>MGHHHHHHENLYFQGHFVQQKVKVFRAADPLVGVFLWGVAHSINELSQVPPPVMLLPDDFKASSKIKVNNHLFHRENLPSHFKFKEYCPQVFRNLRDRFGIDDQDYLVSLTRNPPSESEGSDGRFLISYDRTLVIKEVSSEDIADMHSNLSNYHQYIVKCHGNTLLPQFLGMYRVSVDNEDSYMLVMRNMFSHRLPVHRKYDLKGSLVSREASDKEKVKELPTLKDMDFLNKNQKVYIGEEEKKIFLEKLKRDVEFLVQLKIMDYSLLLGIHDIIRGSEPEEELGPGEFESFIDVYAIRSAEGAPQKEVYFMGLIDILTQYDAKKKAAHAAKTVKHGAGAEISTVHPEQYAKRFLDFITNIFA[2x]

Phosphatidylinositol 5-phosphate 4-kinases (PI5P4Ks) reduce the cellular PI5P pool, using this substrate to generate PI(4,5)P2,12 which has also been shown to be required for successful autophagosome-lysosome fusion. Mammals express three isoforms (α, β, and γ) of PI5P4Ks which have differing tissue specificity and subcellular localization. Variation in catalytic site and putative G-loop sequences may account for the large differences in intrinsic in vitro kinase activity between the isoforms (PI5P4Kγ being 2000-fold less active than PI5P4Kα),19,20 although these differences may be attenuated in vivo. The α, β, and γ subtypes of PI5P4K have almost identical active site residues, with the most significant change being a methionine in PI5P4Kγ (M203) replacing a threonine in PI5P4Kβ (T201) and PI5P4Kα (T196).

To solve structures of PI5P4Kγ as cocomplexes with examples from this chemical series, a truncated version of human PI5P4Kγ comprising residues His32 to Ala421 was cloned into a bacterial expression vector. In both chains, 15 binds deeply in the hydrophobic cleft that forms the ATP binding site in lipid kinases. However, 15 binds in a position in which the heterocycle is rotated approximately 90° within the plane from the cofactor position. A hydrogen bond is formed between the ring sulfur and the side chain of Asn205 and also between the N1 nitrogen and the main chain NH of Met206. The hydrogen atom attached to C2 makes an aromatic hydrogen bond to the backbone carbonyl of Arg 204. The methyl group extending from the 6-position of the thienylpyrimidine ring makes contact with the side chain of Lys216 and also the phenyl ring of Phe207. The methanesulfonylphenyl moiety then runs deep along the back of the binding cavity, forming mainly hydrophobic interactions with residues Lys152, Met203, Ile373, Asp374, and Leu376. The pocket where the sulfone of 15 is located is lined with lipophilic residues: Val154, Phe185, Leu201, Met203, Ile375, and Leu376. The sulfone does not make clear H-bonding interactions in the crystal structure, although a hydrogen bond with the backbone NH of Ile375 is possible. The activation loop formed from residues 377–402 is disordered.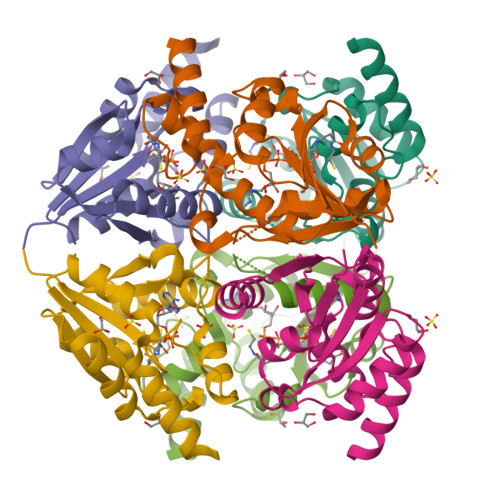> GPGSMVVAVYPGTFDPLTRGHEDLVRRASSIFDTLVVGVADSRAKKPFFSLEERLKIANEVLGHYPNVKVMGFTGLLKDFVRANDARVIVRGLRAVSDFEYEFQMAGMNRYLLPDVETMFMTPSDQYQFISGTIVREIAQLGGDVSKFVFPSVEKWLTEKVAAMAQGPSA> EEVEMAKRRIDEINKELNQVMEQLGDARIDRQESSRQQRKAEIMESIKRLYPGSVYGRLIDLCQPTQKKYQIAVTKVLGKNMDAIIVDSEKTGRDCIQYIKEQRGEPETFLPLDYLEVKPTDEKLRELKGAKLVIDVIRYEPPHIKKALQYACGNALVCDNVEDARRIAFGGHQRHKTVALDGTLFQKSGVISGGASDLKAKARRWDEKAVDKLKEKKGRLTEELLEHHHHHH;> AAKREDLEKKQQLLRAATGKAILNGIDSINKVLEHFRRKGINQHVQNGYHGIVMNNFECEPAFYTCVEVTAGNRLFYHIVDSDEVSTKIL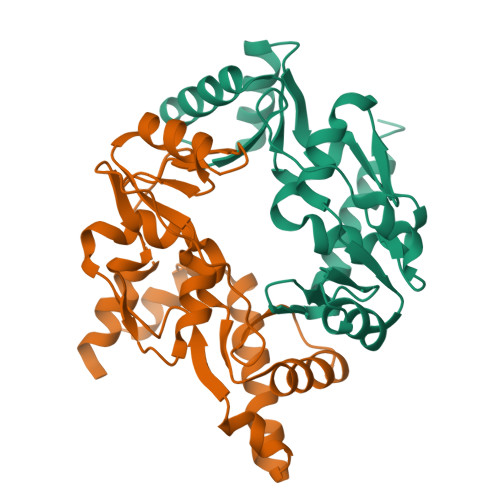MEFNKMNLPGEVTFLPLNKLDVRDTAYPETNDAIPMISKLRYNPRFDKAFKHVFGKTLICRSMEVSTQLARAFTMDCITLEGDQVSHRGALTGGYYDTRKSRLELQKDVRKAEEELGELEAKL>MDKDEAWKQVEQLRREGATRIAYRSDDWRDLKEAWKKGADILIVSSKADDYRARAAAAAKELGNVKPIVDALLAEAKKARDEAWKQVEQLRREGATEIAYRSDDWRDLKEAWKKGADILIVDATDKNEAWKQVEQLRREGATRIAYRSDDWRDLKEAWKKGADILIVDVNARIEKRRKKLAAEGRTDPAVIEAEAAKAREEGWKQVEQLRREGATEIAYRSDDWRDLKEAWKKGADILIVDATLEHHHHHH[2x]

In this work, we diversified a de novo TIM barrel by extending multiple βα‐loops using constrained hallucination. For the diversification experiment, we used the de novo TIM barrel sTIM11‐SB as the base scaffold. This variant contains a stabilizing salt bridge cluster in the lower part of the β‐barrel (Kordes et al., 2022). Here, we introduced two or three helical insertions into minimal loops in the de novo designed TIM barrel sTIM11‐SB.

Within the crystal structure of HalluTIM2‐2, the α‐helical extension at position 1 is resolved entirely; it forms multiple crystal contacts with itself. The second extension at position 3 is not involved in any crystal contacts, and one helical turn before and after the loop could not be resolved. Notably, for both crystal structures, a significant number of crystal contacts are formed within the resolved α‐helices that had been optimized with proteinMPNN. Upon comparison of the obtained crystal structures to corresponding structure predictions using ColabFold, we observed an accurate prediction for HalluTIM2‐2 with a root mean square deviation (RMSD) over all Cα atoms of about 1.2 Å but found major differences in the case of HalluTIM3‐1 as the RMSD over all Cα atoms is over 4.1 Å. In the case of HalluTIM2‐2, the theoretical scatter curves of both the crystal structure and the predicted structure are in overall agreement with the experimental data, with a χ 2 of 2.6 and 2.4, respectively. However, around 0.18 Å−1 both theoretical scatter curves diverge from the experimental data, suggesting a potential high flexibility in the extensions, which is especially conceivable for the partially resolved one. In contrast, in HalluTIM2‐2 and HalluTIM3‐1, a major pocket is formed through the introduced fragments above the C‐terminal end of the inner β‐sheet. These pockets show differences in size with pocket volumes of 1006 Å3 in HalluTIM3‐1 and 2000 Å3 in HalluTIM2‐2.>[2x]MKKILIIGGVAGGASAAARARRLSETAEIIMFERGEYVSFANCGLPYHISGEIAQRSALVLQTPESFKARFNVEVRVKHEVVAIDRAAKLVTVRRLLDGSEYQESYDTLLLSPGAAPIVPPIPGVDNPLTHSLRNIPDMDRILQTIQMNNVEHATVVGGGAIGLEMMESLHHLGIKTTLLELADQVMTPVDREMAGFAHQAIRDQGVDLRLGTALSEVSYQVQT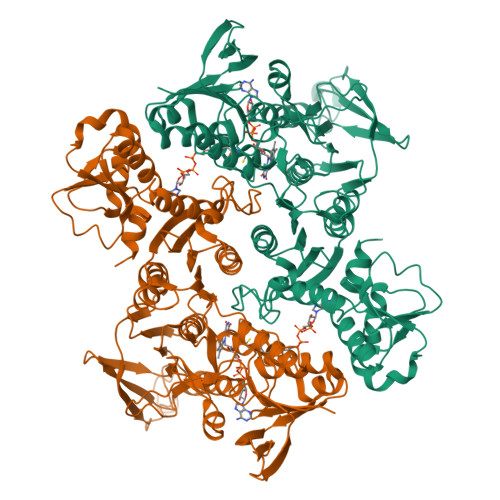HVASDAAGEDTAHQHIKGHLSLTLSNGELLETDLLIMAIGVRPETQLARDAGLAIGELGGIKVNAMMQTSDPAIYAVGDAVEEQDFVTGQACLVPLAGPANRQGRMAADNMFGREERYQGTQGTAICKVFDLAVGATGKNEKQLKQAGIAFEKVYVHTASHASYYPGAEVVSFKLLFDPVKGTIFGAQAVGKDGIDKRIDVMAVAQRAGMTVEQLQHLELSYAPPYGSAKDVINQAAFVASNIIKGDATPIHFDQIDNLSEDQLLLDVRNPGELQNGGLEGAVNIPVDELRDRMHELPKDKEIIIFCQVGLRGNVAYRQLVNNGYRARNLIGGYRTYKFASVLEHHHHHH>MTLIENLNSDKTFLENNQYTDEGVKVYEFIFGENYISSGGLEATKKILSDIELNENSKVLDIGSGLGGGCMYINEKYGAHTHGIDICSNIVNMANERVSGNNKIIFEANDILTKEFPENNFDLIYSRDAILHLSLENKNKLFQKCYKWLKPTGTLLITDYCA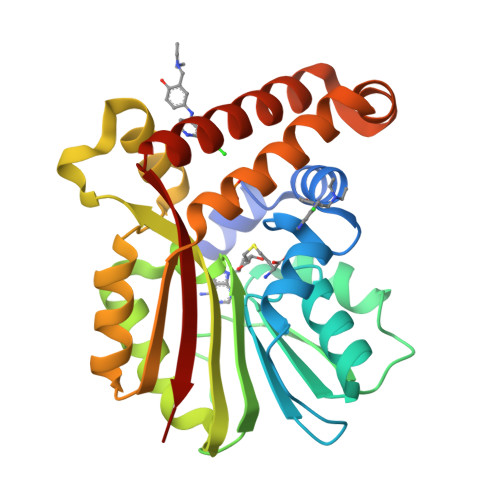TEKENWDDEFKEYVKQRKYTLITVEEYADILTACNFKNVVSKDLSDYWNQLLEVEHKYLHENKEEFLKLFSEKKFISLDDGWSRKIKDSKRKMQRWGYFKATKN[2x]> EKSVSVILLAGGQGKRMKMSMPKQYIPLLGQPIALYSFFTFSRMPEVKEIVVVCDPFFRDIFEEYEESIDVDLSFAIPGKERQDSVYSGL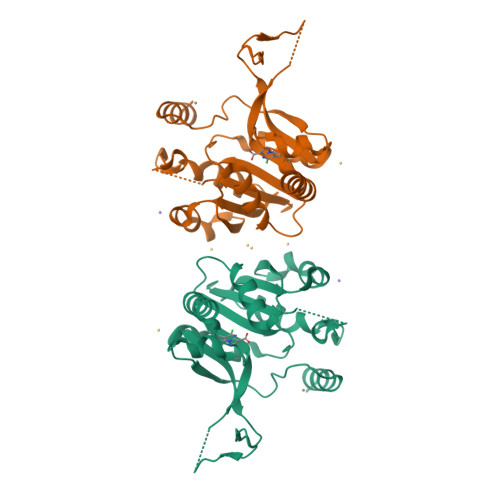QEIDVNSELVCIHDSARPLVNTEDVEKVLKDGSAVGAAVLGVPAKATIKEVNSDSLVVKTLDRKTLWEMQTPQVIKPELLKKGFELVKSEGLEVTDDVSIVEYLKHPVYVSQGSYTNIKVTTPDDLLLAERILSEDS>MQVLNTKSETKQENEGSQPPYIQERLKSLNDIETQLCSMLQEASQVTFIFGELKRGNESVKPQFENHVKQFYERLDKSTTQLRKEIQLLDENVGTRLLPINVNKKALGQDTEKMEEQLDLLSAILDPSKSK[3x];>[3x]MHHHHHHHHHHQRGPGFKFVDLNEKELQNEIKQLGSDSSDGHNSEKKDTDGADENVQIGEDFMEVDYEDKDNPVDSRNETDHKTNENGETDDNIETVMTQEQFVKRRRDMLEHINLAMNESSLALEFVSLLLSSVKESTGMSSMSPFLRKVVKPSSLNSDKIPYVAPTKKEYIELDILNKGWKLQSLNESKDLLRASFNKLSSILQNEHDYWNKIMQSISNKDVIFKIRDRTSGQKLLAIKYGYEDSGSTYKHDRGIANIRNNIESQNLDLIPHSSSVFKGTDFVHSVKKFLRVRIFTKIESEDDYILSGESVMDRDSESEEAETKDIRKQIQLLKKIIFEKELMYQIKKECALLISYGVSIENENKVIIELPNEKFEIELLSLDDDSIVNHEQDLPKINDKRANLMLVMLRLLLVVIFKKTLRSRISSPHGLINLNVDDDILIIRPILGKVRFANYKLLLKKIIKDYVLDIVPGSSITETEVEREQPQENKNIDDENITKLNKEIRAFDKLLNIPRREXXXXXXXXXXXXXXXXXXXXXXXXXXXXXXXXXXXXXXXXXXXXXEVEDFLHFIVAEYIQQKKV;>[3x]MSQSTASLVPEGNQGSLQEDVSFDFNGVPGQALDAVRMRLAQLTHSLRRIRDEMSKAELPQWYTLQSQLNVTLSQLVSVTSTLQHFQETLDSTVVYPLPKFPTTSHESLVTTLLRKKNIPEVDEWMKYVRETSGVTTALLKDEEIEKLLQQDREITNWARTTFRNEYGKHDFKNEESLSEEHASLLVRDSKPSKPFNVDDVLKFTFTGEKPIITGSTSTSSSN;>[3x]MSNQALYEKLEQTRTILSVKLAELINMTTIADRNDDDEGSFAQENSELAVATTSVMMVNNQTMQLIKNVQDLLILTRSIKEKWLLNQIPVTEHSKVTRFDEKQIEELLDNCIETFVAEKTT;>MVQQLSLFGSIGDDGYDLLISTLTTISGNPPLLYNSLCTVWKPNPSYDVENVNSRNQLVEPNRIKLSKEVPFSYLIDETMMDKPLNFRILKS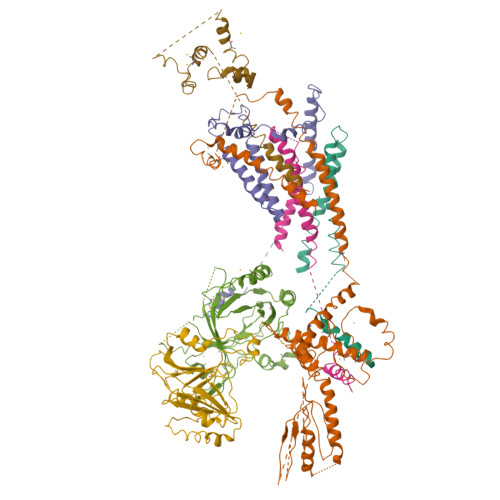FTNDKIPLNYAMTRNINSDDIIDVDMDASPAPSNESCSPWSLQISDIPAAGNNRSVSMQTIAETIILSSAGKNSSVSSLMNGLGYVFEFQYLTIGVKFFMKHGLILELQKIWQIEEAGNSQITSGGFLLKAYINVSRGTDIDRINYTETALMNLKKELQGYIELSVPDRQSMDSRVAHGNILI[3x];>[3x]MGKSAVIFVERATPATLTELKDALSNSILSVRDPWSIDFRTYRCSIKNLPADVSKLMYSITFHHHGRQTVLIKDNSAMVTTAAAADIPPALVFNGSSTGVPESIDTILSSKLSNIWMQRQLIKGDAGETLILDGLTVRLVNLFSSTGFKGLLIELQADEAGEFETKIAGIEGHLAEIRAKEYKTSSDSLGPDTSNEICDLAYQYVRALEL;>[3x]MNVTPLDELQWKSPEWIQVFGLRTENVLDYFAESPFFDKTSNNQVIKMQRQFSQLNDPNAAVNMTQNIMTLPDGKNGNLEEEFAYVDPARRQILFKYPMYMQLEEELMKLDGTEYVLSSVREPDFWVIRKQRRTNNSGVGSAKGPEIIPLQDYYIIGANIYQSPTIFKIVQSRLMSTSYHLNSTLESLYDLIEFQPSQGVHYKVPTDTSTTATAATNGNNAGGGSNKSSVRPTGGANMATVPSTTNVNMTVNTMGTGGQTIDNGTGRTGNGNMGITTEMLDKLMVTSIRSTPNYI>[10x]GPGSMTYLQESSRPAVTVPKLQAMREAGEKIAMLTCYDASFAALLDRANVDVQLIGDSLGNVLQGQTTTLPVTLDDIAYHTACVARAQPRALIVADLPFGTYGTPADAFASAVKLMRAGAQMVKFEGGEWLAETVRFLVERAVPVCAHVGLTPQSVHAFGGFKVQGKTEAGAAQLLRDARAVEEAGAQLIVLEAVPTLVAAEVTRE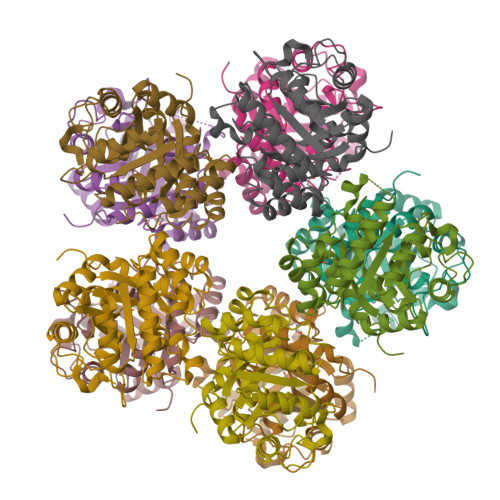LSIPTIGIGAGAECSGQVLVLHDMLGVFPGKRPRFVKDFMQGQPSIFAAVEAYVRAVKDGSFPGPEHSF>ADVIMYEDDHILVLNKPSGTAVHGGSGLSFGVIEGLRALRPEARFLELVHRLDRDTSGVLLVAKKRSALRSLHEQLREKGMQKDYLALVRGQWQSHVKSVQAPLLKNILQSGERIVRVSQEGKPSETRFKVEE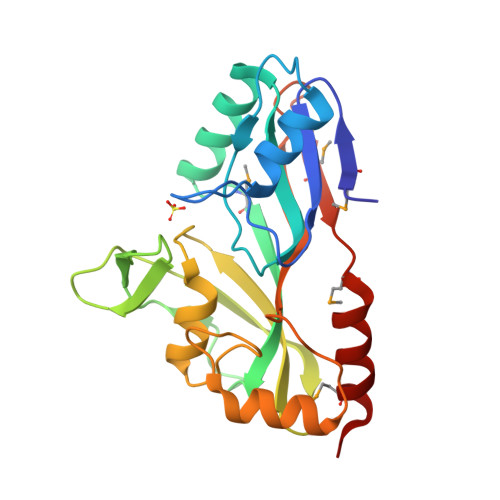RYAFATLVRCSPVTGRTHQIRVHTQYAGHPIAFDDRYGDREFDRQLTEAGTGLNRLFLHAAALKFTHPGTGEVMRIEAPMDEGLKRCLQKMRNAR[2x]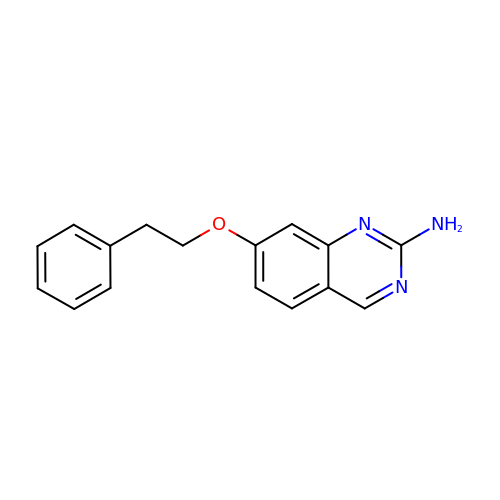7-(2-phenylethoxy)quinazolin-2-amine | C16 H15 N3 O | OERLCDQFGMSRQW-UHFFFAOYSA-N5-BROMO-N[2-(DIMETHYLAMINO)ETHYL]-9-AMINOACRIDINE-4-CARBOXAMIDE | C18 H21 Br N4 O | 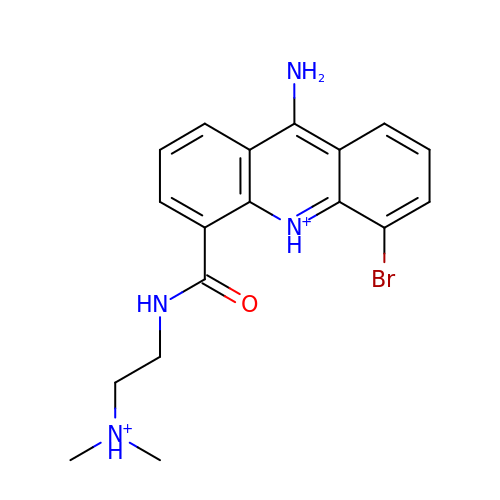NROQPXQSDDINMC-UHFFFAOYSA-P>MLDDAHSLRCNLTIKAPTPADPLWYEAKCLVDEILILHLSNINKTMTSGDPGETANATEVGECLTQPVNDLCQKLRDKVSNTKVDTHKTNGYPHLQVTMIYPQSQGQTPSATWEFNISDSYFFTFYTENMSWRSANDESGVIMNKWNDDGDLV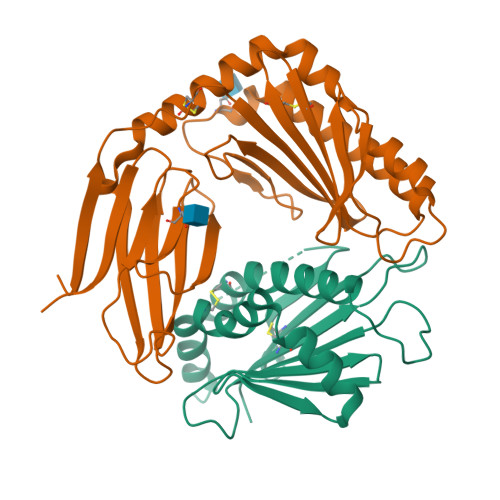QRLKYFIPECRQKIDEFLKQSKEKPRSTSRSPSITQLTSTSPLPPPSHSTSK[2x];>GSSYMDVRIFEDERVDICQDLTATFISYREGPEMFRHSINLEQSSDIFRIEASGEVKHFPWMNVSELAQESAFFVEQERFVYEYIMNVFKAGRPVVFEYRCKFVPFECTVLQMMDGNTLTRYTVDKGVETLGSPPYSPDVSEDDIARYGQGSGISILRDNAALLQKRWTSFCRKIVAMDNPRHNEYSLYSNRGNGYVSCTMRTQVPLAYNISLANGVDIYKYMRMYSGGRLKVEAWLDLRDLNGSTDFAFVISSPTGWYATVKYSEYPQQSPGMLLSSIDGQFESSAVVSWHRGHGLKHAPPVSAEYSILVPRGSHHHHHH[2x]>MDSLAEVEEKYKKAMVSNAQLDNEKTNFMYQVDTLKDMLLELEEQLAESRRQYEEKNKEFEREKHAHSILQFQFAEVKEALKQREEMLE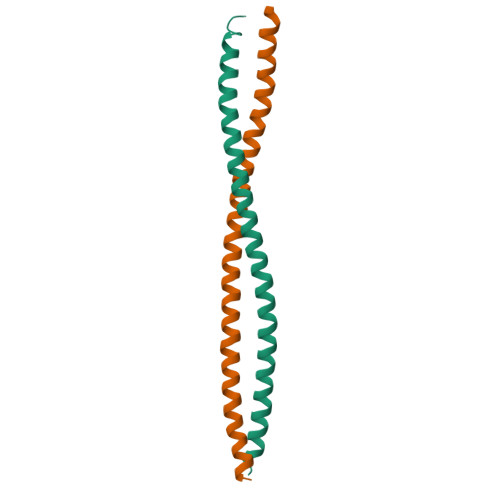PKLAAALEHHHHHH[4x]>[2x]MGPDDYVPSQIAVNTSTLPGVVIGPADAHTYPRVIGELAGTSNQYVFNGGAIALMRGKFTPALPKIGSITYTFHQGNSRDSSDFDIYDIGVSGLGIIIGMAGYWPATPLVPINSSGIYIDPVGANTNPNTYNGATASFGARLFVAFVATGRLPNGYITIPTRQLGTILLEAKRTSLNNKGLTAPVMLNGGRIQVQSQTCTMGLEHHHHHH

Ucl fimbriae are attachment organelles that facilitate ExPEC adherence. Ucl fimbriae are phylogenetically related to Uca fimbriae from Proteus mirabilis and F17/G fimbriae from enterotoxigenic E. coli (ETEC). Tip adhesins are two-domain proteins; they possess a C-terminal pilin domain that connects the adhesin to the main fimbrial shaft, and an N-terminal lectin domain that mediates attachment to specific ligands, therefore dictating host range and tissue tropism.

Next, we determined the crystal structure of UclDLD from F11 at 2.2 Å resolution. At the time of collecting our data, there was no structural model with sufficient sequence identity available in the PDB. Thus, we used iodide SAD phasing, using a sodium iodide derivative of UclDLD that diffracted to 2.85 Å resolution, to obtain phase information. The final UclDLD and UcaDLD models contain residues 21–215 and 21–217, respectively. Electron density was not observed for residues 43–48 (UclDLD) and 44–47 (UcaDLD), suggesting that these regions have a disordered or flexible conformation in the crystals. As expected from the high sequence identity, the two structures are similar, with r.m.s.d. of 0.6 Å for 189 equivalent Cα atoms. UclDLD and UcaDLD have a completely conserved pocket in the same region of the structure as the N-acetylglucosamine (GlcNAc)-binding site in F17G. Of the 358 glycan structures present on the array, UclDLD bound specifically to four glycans. Overall, SPR analyses revealed the strongest binding interaction occurred between UclDLD and sialyllacto-N-fucopentose VI (KD = 11.72 nM ± 3.6). In particular, the swap of asparagine 192 in UcaDLD to a positively charged lysine residue in UclDLD could be the reason for the increased binding affinity for sialyllacto-N-fucopentose VI via its negatively charged sialic acid.> ETGKPSFVTFRGEPAEGFNHLVVDERTGHIYLGAVNRIYKLSSDLKVLVTHQTGPDEDNPKCYPPRIVQTCNEPLASTNNVNKMLLIDYKENRLIACGSLYQGICKLLRLEDLFKLGEPFHKKEHYLSGVNESGSVFGVIVSYSNFDDKLFIATAVDGKPEYFPTISSRKLTKNSEADGMFAYVFHDEFVASMIKIPSDTFTVIPDFDIYYVYGFSSGNFVYFLTLQPEMVSPPGSTTKEQVYTSKLVRLCKEDTAFNSYVEVPIGCERNGVEYRLLQAAYLSKAGAVLGRTLGVRPDDDLLFTVFSKGQKRKMKSLDESALCIFILKQINDRIKDRLQSCYRGEGTLDLAWLKVKDIPCSSALLTIDDNFCGLDMNAPLGVSEMVRGIPVFTEDRDRMTSVIAYVYKNHSLAFVGTKSGKLKKIRVDGPKGNALQYETVQVVDSGPVLRDMAFSKDHEQLYIMSERQLTRVPVESCGQYRSCGECLGSGDPHCGWCVLHNTCTRKERCERSREPRRFASEMKQCVRLTVHPNNISVSQYNVLLVLETYNVPELSAGVNCTFEDLSEMDGLVIGNQIQCYSPAAKEVPRIITENGDHHVVQLQLKSKETGMTFASTSFVFYNCSVHNSCLSCVESPYRCHWCKYRHVCTHDPNTCSFQEGRVKLPEDCPQLLRVDKILVPVEVIKPITLKAKNLPQPQSGQRGYECILNIQGIEQRVPALRFNSSSVQCQNTSY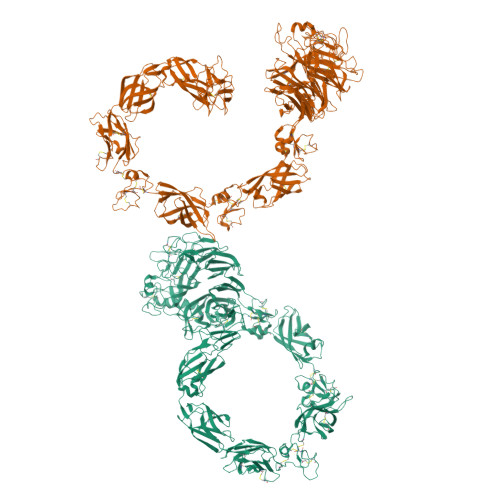SYEGMEINNLPVELTVVWNGHFNIDNPAQNKVYLYKCGAMRESCGLCLKADPDFECGWCQSPGQCTLRQHCPAHESRWLELSGANSKCTNPRITEIIPVTGPREGGTKVTIRGENLGLEFRDIASHVKVAGVECSPLVDGYIPAEQIVCEMGEAKPSQHAGFVEICVAVCRPEFMARSSQLYYFMTLTLADLKPNRGPMSGGTQVTITGTNLNAGSNVVVMFGSQPCLFHRRSPSYIICNTTSSEEVLDMKVTVQVDRARIRQDLVFQYVEDPTIVRIEPEWSIVSGNTPIAVWGTHLDLIQNPQIRAKHGGKEHINICEVLNATEMTCQAPALALGPDHQSDLTERPEEFGFILDNVQSLLILNKTNFTYYPNPVFEAFSPSGILELKPGTPIILKGKNLIPPVAGGNVKLNYTVLVGEKPCTVTVSDVQLLCESPNLIGRHKVMARVGGMEYSPGMVYIAPGRTKHHHHHH>MTDYDKLSNLATTFEFPDLTVEIKGPDVVGVNKLAEYEV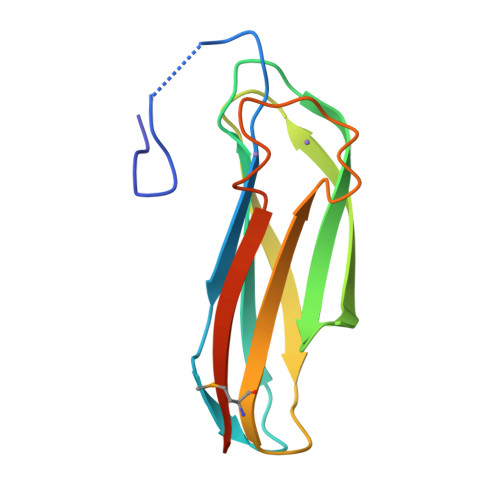HVKNLGGIGVPSTKVRVYINGTLYKNWTVSLGPKEEKVLTFNWTPTQEGMYRINATVDEENTVVELNENNNVATFDVSVVLEHHHHHH[2x]>[4x]MGNSIKTLSNLANLLAQEGKAEEAIKYMRKAVSLDPNNIKTLSNLANLLAQEGKAEEAIKYMRKAVSLDPNNIKTLSNLAVLLAQEGKAEEAIKYMRKAVSLIDKAAKG

One of these highly populated repetitive folds is the αα-solenoid (SCOP a.118), whose most widespread superfamily is the tetratricopeptide repeat (TPR; a.118.8). The ﬁrst crystal structure of a TPR domain showed that the repeat units are helical hairpins, stacked into a continuous, right-handed superhelical architecture with an inner groove that mediates the interaction with target proteins. Here we show that such hairpins are detectable and that one of them, from the ribosomal protein RPS20, can be customized to yield a TPR fold by repetition, with only a small number of point mutations that are neutral for the parent organism. We concatenated three copies of RPS20-hhta as an initial construct, connected by the TPR consensus loop sequence (DPNN).

M4NΔC is M4N without stop helix. We conclude that in the amplified constructs, the observed interactions are more favorable than the interaction with the native stop helix, releasing it and rendering it prone to degradation. This led us to ask whether this helix is in fact dispensable. Indeed, an M4NΔC construct, which terminates with the B3 helix, showed the same stability and dimerization as M4N. We obtained two structures for M4NΔC from different crystal forms at 2.0 Å and 1.7 Å resolution, respectively, the first (CF I) with two dimers in the ASU and the second (CF II) with a single chain in the ASU, for which we constructed the dimer by crystallographic symmetry. (a) Two dimers in the ASU of M4NΔC CF I. (b) Dimer constructed by applying the crystallographic symmetry to the single chain in the ASU of M4NΔC CF II. All three dimers superimpose to the M4N dimer with Cα RMSD below 1.9 Å.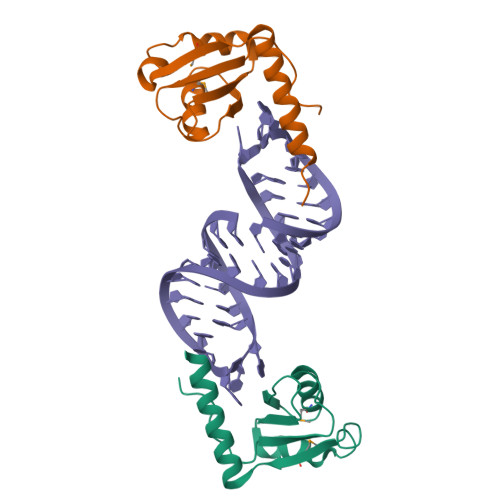>[2x]SNATGPQFVSGVIVKIISTEPLPGRKQVRDTMAAISEVLYVDLLEGDTECHARFKTPLDALAVINAYTEINKKHCWKMEILSGDHEQRYWQKILVDRQAKLNQPREKKRGTEK> MAPFRQDSILIIYPRSQTTLVQFGLNEETFTVPELEIPTQIYRTTRQDGSYTYHSTNKDNKAELIKPIQNGEIIDISAFTQFLRLIFVSILSDRANKNQDAFEAELSNIPLLLITHHSWSQSDLEIITQYVFESLEINNLIQLPASLAATYSMISLQNCCIIDVGTHHTDIIPIVDYAQLDHLVSSIPMGGQSINDSLKKLLPQWDDDQIESLKKSPIFEVLSDDAKKLSSFDFGNENEDEDEGTLNVAEIITSGRDTREVLEERERGQKVKNVKNSDLEFNTFWDEKGNEIKVGKQRFQGCN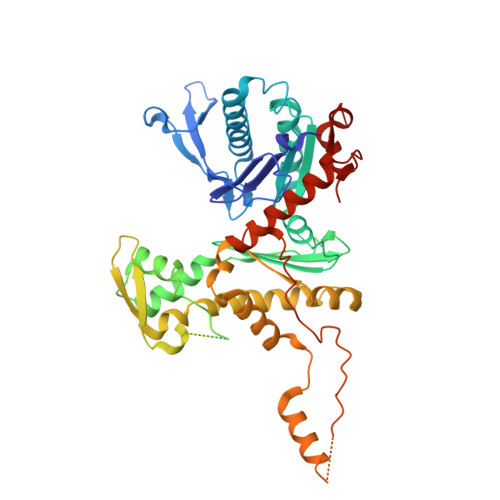NLIKNISNRVGLTLDNIDDINKAKAVWENIIIVGGTTSISGFKEALLGQLLKDHLIIEPEEEKSKREEEAKSVLPAATKKKSKFMTNSTAFVPTIEYVQCPTVIKLAKYPDYFPEWKKSGYSEIIFLGAQIVSKQIFTHPKDTFYITREKYNMKGPAALWDVQF>[2x]DMDLDSYQIALEEVLTWLLSAEDTFQEQDDISDDVEDVKEQFATHETFMMELSAHQSSVGSVLQAGNQLMTQGTLSDEEEFEIQEQMTLLNARWEALRVESMERQSRLHDALMELQKK

Dystrophin is a large (427 kD) multidomain protein expressed in skeletal and cardiac muscle where it binds to the dystrophin-associated glycoprotein (DAG) complex of the plasma membrane and to F-actin connecting the cytoskeleton to the membrane. Utrophin (Utr), the 395 kD autosomal homologue of Dys is widely expressed in non muscle tissues (reviewed) but is restricted to the myotendinous and neuromuscular junctions of differentiated muscle and is located at the sarcolemma of developing fetal muscle. Dys and Utr potentially act as cellular biomechanical shock-absorbers limiting damage to the plasma membrane with the spectrin repeat domains acting as spring units by undergoing force-induced unfolding. Dys and Utr-SR1 adopt the canonical spectrin repeat fold comprising a triple helical bundle displaying an approximately cylindrical structure of overall dimensions ∼60 Å length and ∼9 Å radius (between backbone atoms).

The Utr N-terminal spectrin repeat 1 (Utr-SR1) crystallised with two molecules in the asymmetric unit of the P212121 cell and has been refined to a final model with crystallographic R and Rfree values of 0.200 and 0.235 with diffraction data of outer limit 1.95 Å resolution. Helix A (Utr 310–334; Dys 340–364, residue number is offset by +30 for Dys-SR1 relative to Utr-SR1) is shorter than B (Utr 342–379; Dys 372–409) and C (Utr 384–423; Dys 414–453) with the triple helix structure changing to coiled-coil formed between the B and C helices after the C-terminal end of helix A, a conserved feature for spectrin repeats domains. Helices A and C are straight but helix B has an appreciable bend in the centre with the loss of canonical main chain n+4 helical hydrogen bonding for residues Utr 360–361.This bending of helix B, a conserved spectrin repeat domain structural motif, is stabilised by conserved side chain stacking interactions between H362 and W324 (helix A) in combination with W401 (helix C) augmenting the hydrophobic heptad repeat central domain core. H362 is not strictly conserved for Utr/Dys or homologous repeats often replaced by Pro, that is also accommodated within the helix B bend. Analysis of molecular packing in the Utr-SR1 crystal revealed an interaction predicted to be relevant with respect to oligomerisation burying 1260 Å2 surface area between monomers A and B. However size exclusion chromatography data for Utr/Dys-SR1, as well as previous studies, show that Utr (and Dys) are monomeric suggesting that the degree of association observed in the crystal is most likely owing to crystal packing and the non-globular nature of the SR tertiary structure. Curiously the Utr-SR1 (and Utr-SR1-L) structures are the first single spectrin repeat structures determined by x-ray crystallography in the Protein Data Bank; the single drosophila α-spectrin repeat 14 structure has been determined but crystallizes in a domain-swapped dimer conformation rather than the isolated three-helix bundle fold and Dys-SR1 is disulphide linked.>[4x]MNYQNDDLRIKEIKELLPPVALLQKFPATENAANTVAHARKAIHKILKGNDDRLLVVIGPCSIHDPVAAKEYATRLLALREELKDELEIVMRVYFEKPRTTVGWKGLINDPHMDNSFQINDGLRIARKLLLDINDSGLPAAGEFLDMITPQYLADL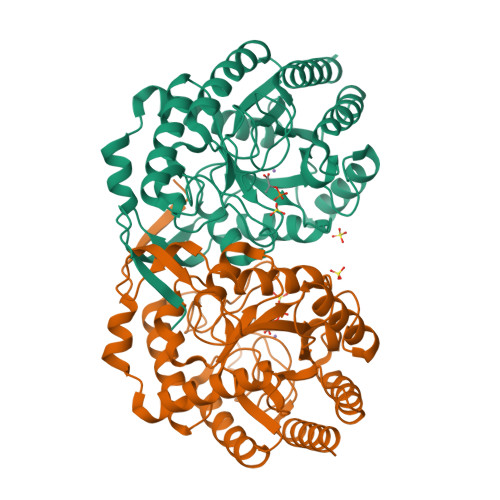MSWGAIGARTTESQVHRELASGLSCPVGFKNGTDGTIKVAIDAINAAGAPHCFLSVTKWGHSAIVNTSGNGDCHIILRGGKEPNYSAKHVAEVKEGLNKAGLPAQVMIDFSHANSSKQFKKQMDVCADVCQQIAGGEKAIIGVMVESHLVEGNQSLESGEPLAYGKSITDACIGWEDTDALLRQLANAVKARRG>GMQIESFKSLLPKYKCIFFDAFGVLKTYNGLLPGIENTFDYLKAQGQDYYIVTNDASRSPEQLADSYHKL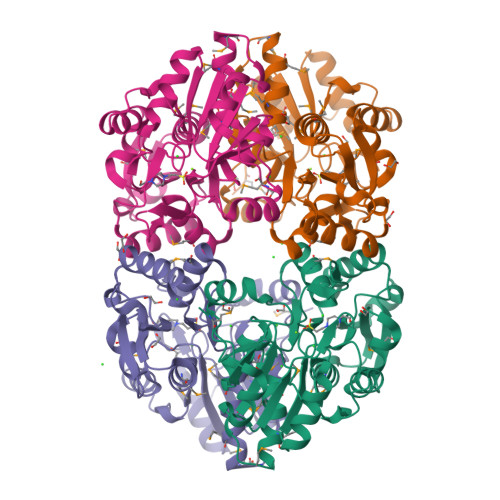GLFSITADKIISSGMITKEYIDLKVDGGIVAYLGTANSANYLVSDGIKMLPVSAIDDSNIGEVNALVLLDDEGFNWFHDLNKTVNLLRKRTIPAIVANTDNTYPLTKTDVAIAIGGVATMIESILGRRFIRFGKPDSQMFMFAYDMLRQKMEISKREILMVGDTLHTDILGGNKFGLDTALVLTGNTRIDDAETKIKSTGIVPTHICESAVIEL[4x]>GSMLKLRQLQKKKQKENENSSSIQPNLSAARIRLKRDLDSLDLPPTVTLNVITSPDSADRSQSPKLEVIVRPDEGYYNYGSINFNLDFNEVYPIEPPKVVCLKKIFHPNIDLKGNVCLNILREDWSPALDLQSIITGLLFLFLEPNPNDPLNKDAAKLL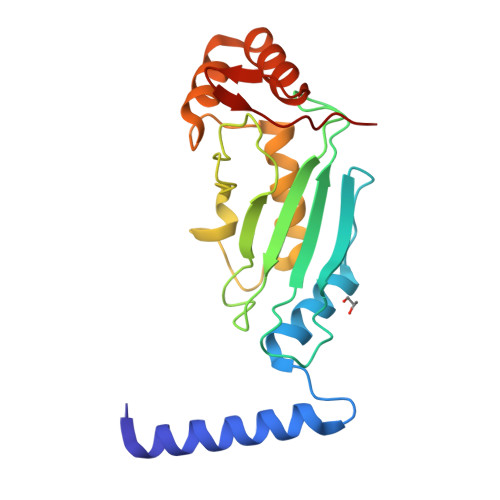CEGEKEFAEAVRLTMSGGSIEHVKYDNIVSP[2x]>MDLPKAYDPKSVEPKWAEKWAKNPFVANPKSGKPPFVIFMPPPNVTGSLHMGHALDNSLQDALIRYKRMRGFEAVWLPGTDHAGIATQVVVERLLLKEGKTRHDLGREKFLERVWQWKEESGGTILKQLKRLGASADWSREAFTMDEKRSRAVRYAFSRYYHEGLAYRAPRLVNWCPRCETTLSDLEVETEPTPGKLYTLRYEVEGGGFIEIATVRPETVFADQAIAVHPEDERYRHLLGKRARIPLTEVWIPILADPAVEKDFGTGALKVTPAHDPLDYEIGERHGLKPVSVINLEGRMEGERVPEALRGLDRFEARRKAVELFREAGHLVKEEDYTIALATCSRCGTPIEYAIFPQWWLRMRPLAEEVLKGLRRGDIAFVPERWKKVNMDWLENVKDWNISRQLWWGHQIPAWYCEDCQAVNVPRPERYLEDPTSCEACGSPRLKRDEDVFDTWFSSALWPLSTLGWPEETEDLKAFYPGDVLVTGYDILFLWVSRMEVSGYHFMGERPFKTVLLHGLVLDEKGQKMSKSKGNVIDPLEMVERYGADALRFALIYLATGGQDIRLDLRWLEMARNFANKLYNAARFVLLSREGFQAKEDTPTLADRFMRSRLSRGVEEITALYEALDLAQAAREVYELVWSEFCDWYLEAAKPALKAGNAHTLRTLEEVLAVLLKLLHPMMPFLTSELYQALTGKEELALEAWPEPGGRDEEAERAFEALKQAVTAVRA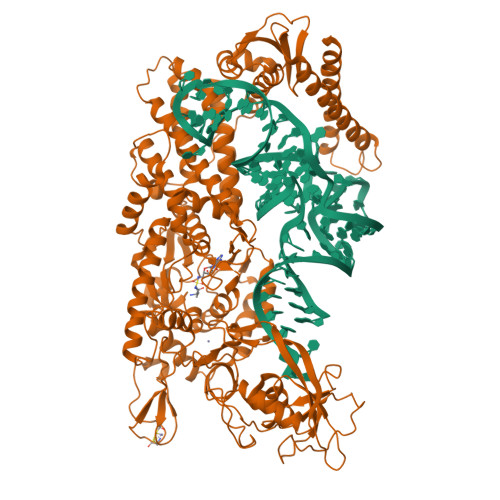LKAEAGLPPAQEVRVYLEGETAPVEENLEVFRFLSRADLLPERPAKALVKAMPRVTARMPLEGLLDVEEWRRRQEKRLKELLALAERSQRKLASPGFREKAPKEVVEAEEARLKENLEQAERIREALSQIG[2x]> MISVNDFKTGLTISVDNAIWKVIDFQHVKPGKGSAFVRSKLRNLRTGAIQEKTFRAGEKVEPAMIENRRMQYLYADGDNHVFMDNESFEQTELSSDYLKEELNYLKEGMEVQIQTYEGETIGVELPKTVELTVTETEPGIKGDTATG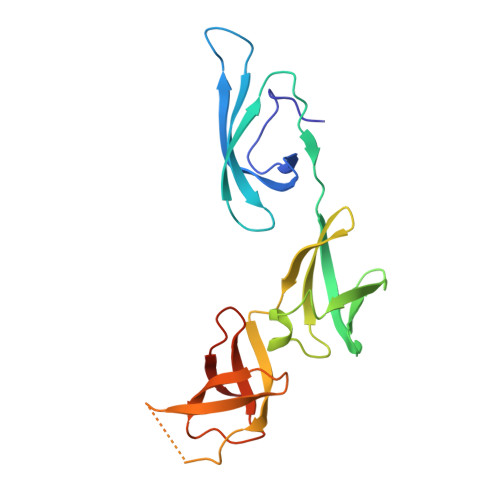ATKSATVETGYTLNVPLFVNEGDVLIINTGDGSYISRGHHHHHH> GHMAAAAELSLLEKSLGLSKGNKYSAQGERQIP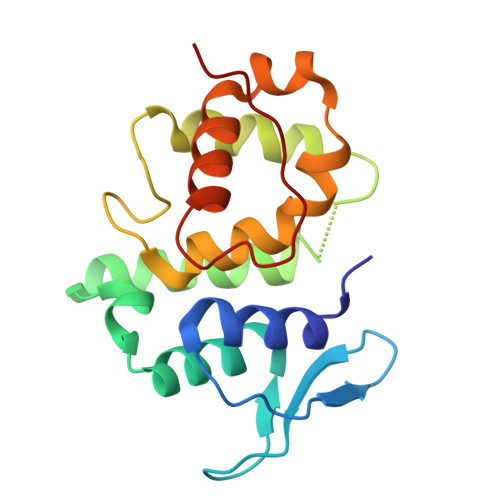VLQTNNGPSLTGLTTIAAHLVKQANKEYLLGSTAEEKAIVQQWLEYRVTQVDGHSSKNDIHTLLKDLNSYLEDKVYLTGYNFTLADILLYYGLHRFIVDLTVQEKEKYLNVSRWFCHIQHYPGIRQHLSSVVFIKNRL> ATGGYVQQATGQASFTMYSGCGSPACGKAASGFTAAINQLAFGSAPGLGAGDACGRCFALTGNHDPYSPNYTGPFGQTIVVKVTDLCPVQGNQEFCGQTTSNPTDQHGMPFHFDICEDTGGSAKFFPSGHGAL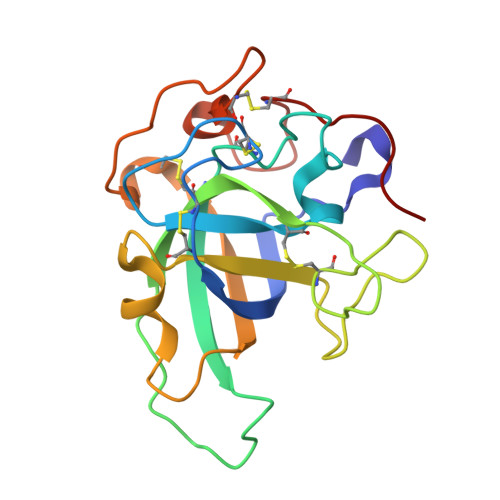TGTFTEVSCSQWSGSDGGQLWNGACLSGETAPNWPSTACGNKGTAPS>[4x]MTSSKIEMPGEVKADPAALMASLHLLPSPTPNLEIKYTKIFINNEWQNSESGRVFPVYNPATGEQVCEVQEADKADIDKAVQAARLAFSLGSVWRRMDASERGRLLDKLADLVERDRAVLATMESL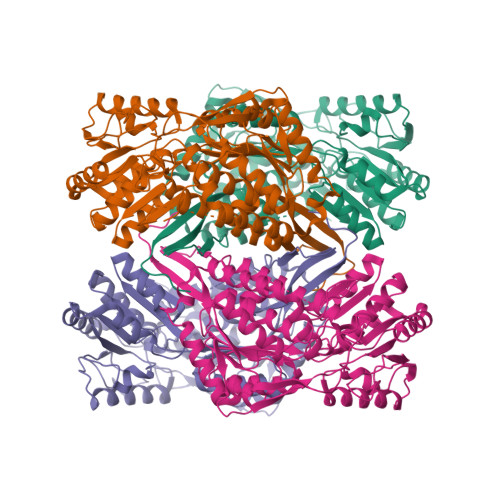NGGKPFLQAFYVDLQGVIKTFRYYAGWADKIHGMTIPVDGDYFTFTRHEPIGVCGQIIPWNFPLLMFAWKIAPALCCGNTVVIKPAEQTPLSALYMGALIKEAGFPPGVINILPGYGPTAGAAIASHIGIDKIAFTGSTEVGKLIQEAAGRSNLKRVTLELGGKSPNIIFADADLDYAVEQAHQGVFFNQGQCCTAGSRIFVEESIYEEFVRRSVERAKRRVVGSPFDPTTEQGPQIDKKQYNKILELIQSGVAEGAKLECGGKGLGRKGFFIEPTVFSNVTDDMRIAKEEIFGPVQEILRFKTMDEVIERANNSDFGLVAAVFTNDINKALTVSSAMQAGTVWINCYNALNAQSPFGGFKMSGNGREMGEFGLREYSEVKTVTVKIPQKNS>MLIPAQENNVSLTATPSRIGQIMKYGFPGLDHVRSHSDYVLSYDRRNRVPHWVFEHLTAESVAKNDAVDRSKCDF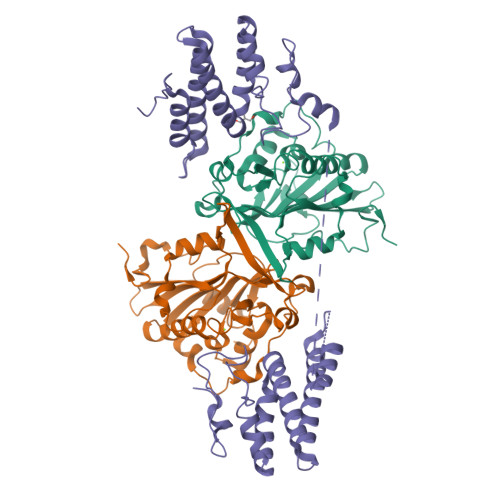KQDESIHPFFRSQNTDYRRSGYDRGHMAAAGNHRLHQKHCDETFYLSNMAPQVGQGFNRDAWNTLEAHVRRLTKTYSNVYVCTGPLYLPHKEDDGKSYVKYEVIGANTVAVPTHFYKVIVGESADHKLHMESYVMPNQVISNDTPISVFQVPPESVERSAGLLFFDQINRKQLTTINGKKVAAALEHHHHHH[2x];> MAKRKAEDTQSDKMATAEKVAQNDYTIGLVDPVKDYQKLIETRVQVDEIVDDDVTKENFDRTAAAARDVIWRLLFDEAGTSQSNTEKASQLLEEYRGDACFYDPTPYNEWIVKLRDEVLKKELLDFWRDVLVKKQLGPCWSRDSDLFDSDDTPPLEFYAHAGCTAPFAASLKVRAALEEQASLDQDGPATPTTPGELSADDAAALSGEFEATLTKENPLEEYRTLMKRFVLTKIIVPDSVHQASVKKIAAAAREIIWKLLFDGTPSAEDQNKAAELLQEYKGDAGFYGPDDYNSWIFNLRDEVLTKELLDFWRDKMVKMELGPSCARDSDYYDNEDPLPFEFYEKAGCKAPFEGPVNDD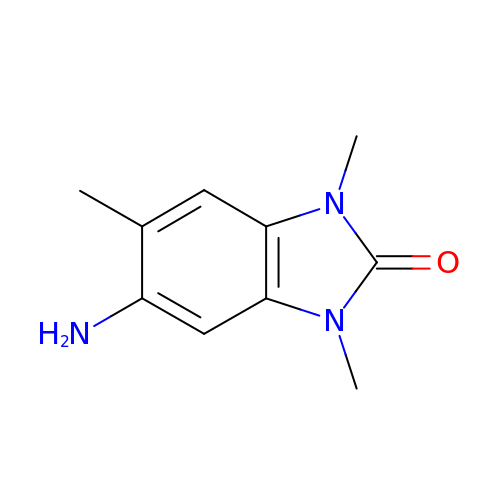5-amino-1,3,6-trimethyl-1,3-dihydro-2H-benzimidazol-2-one | C10 H13 N3 O | DHPXTEFKFUCWDK-UHFFFAOYSA-N>[2x]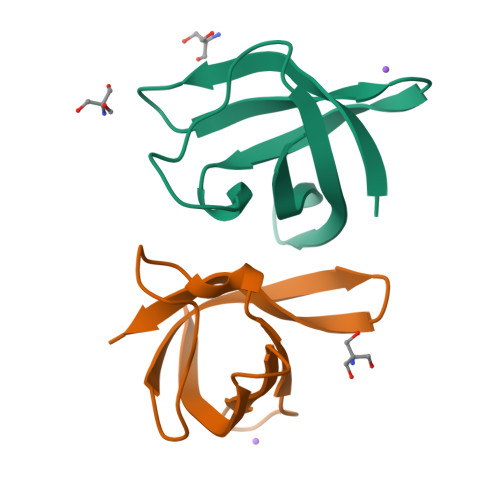MQRGKVKWFNNEKGYGFIEVEGGSDVFVHFTAIQGEGFKTLEEGQEVSFEIVQGNRGPQAANVVKL> RHMTRYDSLLQALGNTPLVGLQRLSPRWDDGRDGPHVRLWAKLEDRNPTGSIKDRPAVRMIEQAEADGLLRPGATILEPTSGNTGISLAMAARLKGYRLICVMPENTSVERRQLLELYGAQIIFSAAEGGSNTAVATAKELAATNPSWVM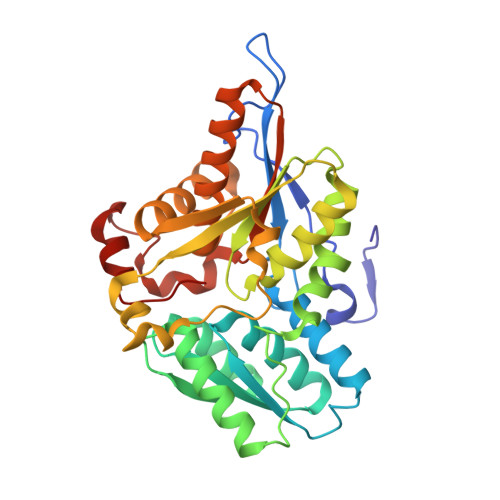LYQYGNPANTDSHYCGTGPELLADLPEITHFVAGLGTTGTLMGTGRFLREHVANVKIVAAEPRYGEGVYALRNMDEGFVPELYDPEILTARYSVGAVDAVRRTRELVHTEGIFAGISTGAVLHAALGVGAGALAAGERADIALVVADAGWKYLSTGAYAGSLDDAETALEGQLWA> PASLTEIEHLVQSVCKSYRETCQLRLEDLLRQRSNIFSREEVTGYQRKSMWEMWERCAHHLTEAIQYVVEFAKRLSGFMELCQNDQIVLLKAGAMEVVLVRMCRAYNADNRTVFFEGKYGGMELFRALGCSELISSIFDFSHSLSALHFSEDEIALYTALVLINAHRPGLQEKRKVEQLQYNLELAFHHHLCKTHRQSILAKLPPKGKLR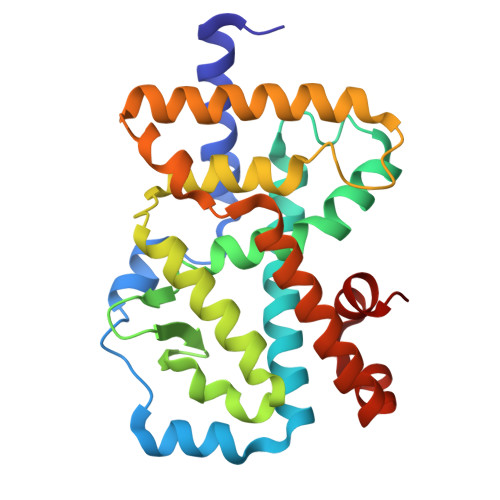SLCSQHVERLQIFQHLHPIVVQAAFPPLYKELFSTE> GSHMSLAIDLEVKQDVLIVRLSGELDHHTAEELREQVTDVLENRAIRHIVLNLGQLTFMDASGLGVILGRYKQIKNVGGQMVVCAVSPAVKRLFDMSGLFKIIRVEADEQFALQALGV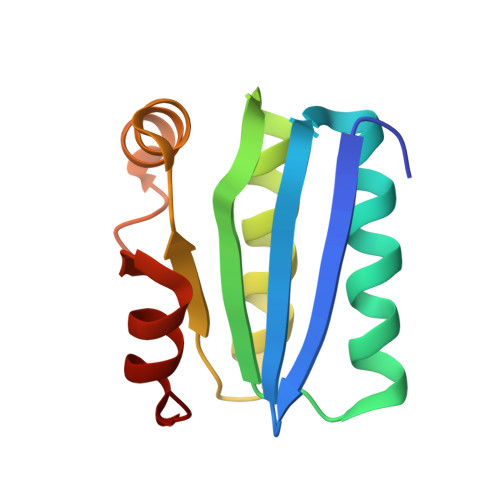A>[6x]VPRPPAPLFRDPIYDGAADPTIIYNHLEKSWWILYTNRRANQKLPGKAFMHGTDIGIAESKDGGRTWFYRGTIELQY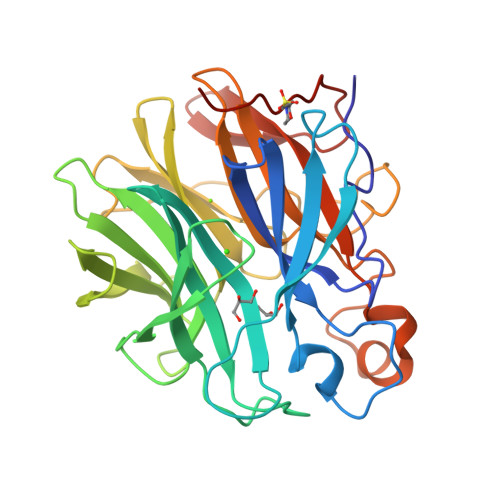GRGRNTFWAPEVIFYEGEYHMYVSFVPGVPQDWNAERYILYYKSKNLWDWEFVCKLELSSNKVIDACVFQMPDGTFRMWYKDEADHSYIYAAESNNLKDWKILGPALTDRPQEGPNVFWWKSKYWMITDPWCGLGVYSSEDATAWHRHENILDRPGKREDDGQIGHHADVLVIDDETAYIFYFTHPEGMEGTEEFWKDSKYWRTSLQVAKLEYVDGKVVCDRDKEFDFYLPDLFAHHHHHH> GSD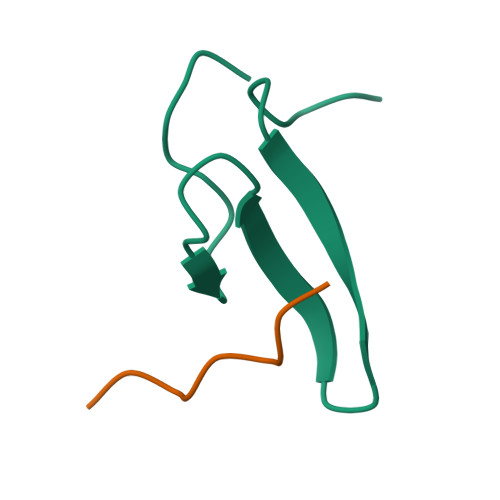LPAGWMRVQDTSGTYYWHIPTGTTQWEPPGRASPS;> PPPPPPLPP>AVKFGWIKGVLVRCMLNIWGVMLFIRLSWIVGQAGIGLSVLVIMMATVVTTITGLSTSAIATNGFVRGGGAYYLISRSLGPEFGGAIGLIFAFANAVAVAMYVVGFAETVVELLKEHSILMIDEINDIRIIGAITVVILLGISVAGMEWEAKAQIVLLVILLLAIGDFVIGTFIPLESKKPKGFFGYKSEIFNENFGPDFREEETFFSVFAIFFPAATGILAGANISGDLADPQSAIPKGTLLAILITTLVYVGIAVSVGSCVVRDATGNVNDTIVTELTNCTSAACKLNFDFSSCESSPCSYGLMNNFQVMSMVSGFTPLISAGIFSATLSSALASLVSAPKIFQALCKDNIYPAFQMFAKGYGKNNEPLRGYILTFLIALGFILIAELNVIAPIISNFFLASYALINFSVFHASLAKSPGWRPAFKYYNMWISLLGAILCCIVMFVINWWAALLTYVIVLGLYIYVTYKKPDVNWGSSTQALTYLNALQHSIRLSGVEDHVKNFRPQCLVMTGAPNSRPALLHLVHDFTKNVGLMICGHVHMGPRRQAMKEMSIDQAKYQRWLIKNKMKAFYAPVHADDLREGAQYLMQAAGLGRMKPNTLVLGFKKDWLQADMRDVDMYINLFHDAFDIQYGVVVIRLKEGLDISHLQGQEELLSSQEKSPGTKDVVVSVEYSKKSDLDTSKPLSEKPITHKVEEEDGKTATQPLLKKESKGPIVPLNVADQKLLEASTQFQKKQG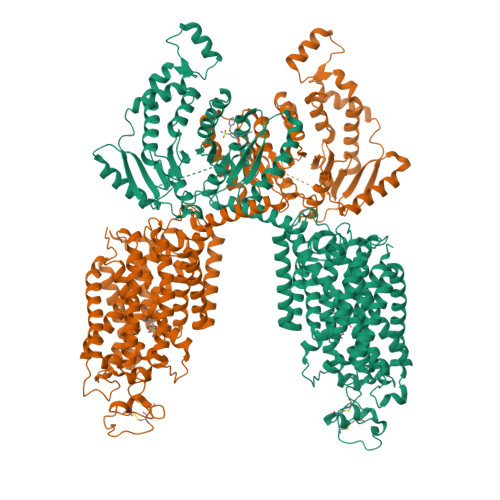KNTIDVWWLFDDGGLTLLIPYLLTTKKKWKDCKIRVFIGGKINRIDHDRRAMATLLSKFRIDFSDIMVLGDINTKPKKENIIAFEEIIEPYRLHEDDKEQDIADKMKEDEPWRITDNELELYKTKTYRQIRLNELLKEHSSTANIIVMSLPVARKGAVSSALYMAWLEALSKDLPPILLVRGNHQSVLTFY[2x]> MRGIVTIDGPSASGKSSVARRVAAALGVPYLSSGLLYRAAAFLALRAGVDPGDEEGLLALLEGLGVRLLAQAEGNRVLADGEDLTSFLHTPEVDRVVSAVARLPGVR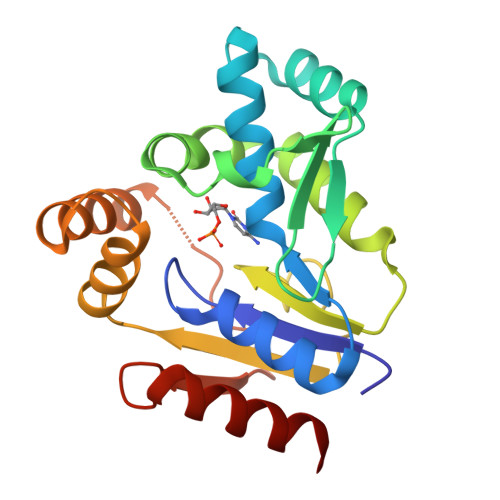AWVNRRLKEVPPPFVAEGRDMGTAVFPEAAHKFYLTASPEVRAWRRARERPQAYEEVLRDLLRRDERDKAQSAPAPDALVLDTGGMTLDEVVAWVLAHIRR> GLVPRGSHMFIMIGERINGMFKDIREAILNKDPRPIQEWARRQAEKGAHYLDVNTG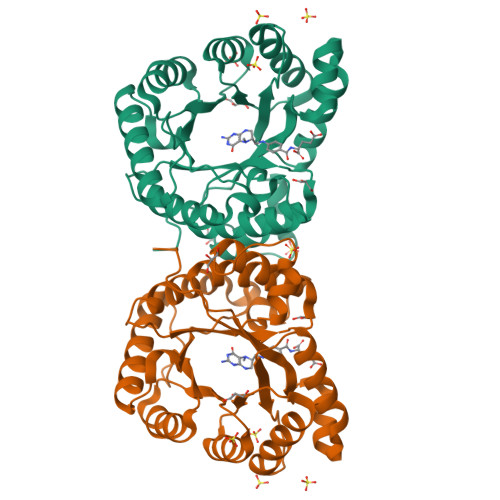PTADDPVRVMEWLVKTIQEVVDLPCCLDSTNPDAIEAGLKVHRGHAMINSTSADQWKMDIFFPMAKKYEAAIIGLTMNEKGVPKDANDRSQLAMELVANADAHGIPMTELYIDPLILPVNVAQEHAVEVLETIRQIKLMANPAPRTVLGLSNVSQKCPDRPLINRTYLVMAMTAGLDAAIMDVDDDALVDAAATAHILLNKEIYCDSYLKTFRQK>[3x]MALYREGKAAMAADGTVTGTGTKWQSSLSLIRPGATIMFLSSPIQMAVVNKVVSDTEIKAITTSGAVVASTDYAILLSDSLTVDGLAQDVAETLRHYQSQETVIADAVEFFKSFDFDSLQNLANQIKADSESAESSAAAAAASESKAKTSEDNAKSSENAAKNSEVAAETTRDQIQQIIDNAGDQSTLVVLAQPDGFDSIGRVSSFAALRNLKPKKSGQHVLLTSYYDGWAAENKMPTGGGEFISSIGTATDDGGYIAAGPGYYWTRVVNNNSFTAEDFGCKTTATPPPNFNVLPAELFDNTAMMQAAFNLAISKSFKLNLSTGTYYFESSDTLRITGPIHIEGRPGTVFYHNPSNKANPKTDAFMNISGCSAGRISSINCFSNSYLGKGINFDRSVGDNRKLVLEHVYVDTF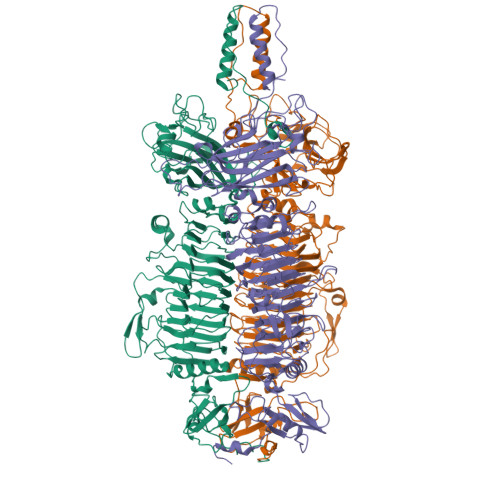RWGFYVGEPECINQIEFHSCRAQSNYFQGIFIESFKEGQEYGHSAPVHFFNTICNGNGPTSFALGATYKTTKNEYIKVMDSVNDVGCQAYFQGLSNVQYIGGQLSGHGSPRNTSLATITQCNSFIIYGTDLEDINGFTTDGTAITADNIDAIESNYLKDISGAAIVVSSCPGFKIDSPHIFKIKTLSTIKLMNNTYNYEIGGFTPDEALKYNVWDANGLATNRISGVIHPRLVNSRLGINSVAFDNMSNKLDVSSLIHNETSQIVGLTPSTGSNVPHTRKMWSNGAMYSSTDLNNGFRLNYLSNHNEPLTPMHLYNEFSVSEFGGSVTESNALDEIKYIFIQTTYANSGDGRFIIQALDASGSVLSSNWYSPQSFNSTFPISGFVRFDVPTGAKKIRYGFVNSANYTGSLRSHFMSGFAYNKRFFLKIYAVYNDLGRYGQFEPPYSVAIDRFRVGDNTTQMPSIPASSATDVAGVNEVINSLLASLKANGFMSS(4~{S})-4-[(1~{R})-1-[(1~{R},3~{a}~{S},4~{E},7~{a}~{R})-7~{a}-methyl-4-[2-[(3~{R},5~{R})-4-methylidene-3,5-bis(oxidanyl)cyclohexylidene]ethylidene]-2,3,3~{a},5,6,7-hexahydro-1~{H}-inden-1-yl]ethyl]-1-(1~{H}-pyrrol-2-yl)octan-1-one 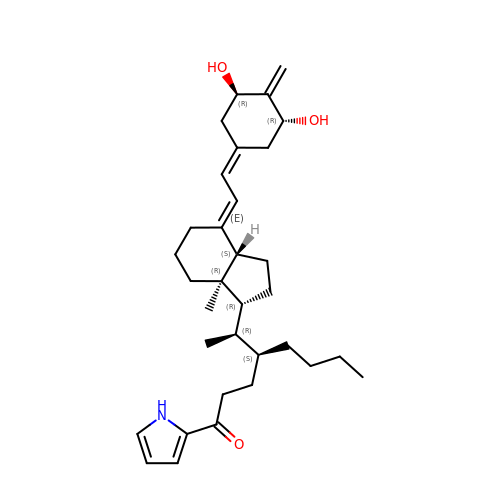| C33 H49 N O3 | LSFVNCITLLLHBJ-LTRSXRPOSA-N> MTENILRKSDEEIQKEITARVKALESMLIEQGILTTSMIDRMAEIYENEVGPHLGAKVVVKAWTDPEFKKRLLADGTEACKELGIGGLQGEDMMWVENTDEVHHVVVCTLCSCYPWPVLGLPPNWFKEPQYRSRVVREPRQLLKEEFGFEVP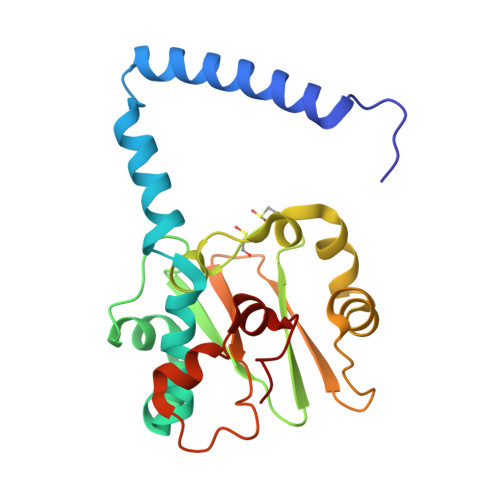PSKEIKVWDSSSEMRFVVLPQRPAGTDGWSEEELATLVTRESMIGVEPAKAVA> PELPEVETIRRTLLPLIVGKTIEDVRIFWPNIIRHPRDSEAFAARMIGQTVRGLERRGKFLKFLLDRDALISHLRMEGRYAVASALEPLEPHTHVVFCFTDGSELRYRDVRKFGTMHVYAKEEADRRPPLAELGPEPLSPAFSPAVLAERAVKTKRSVKALLLDCTVVAGFGNIYVDESLFRAGILPGRPAASLSSKEIERLHEEMVATIGEAVMKGQHHLYVYG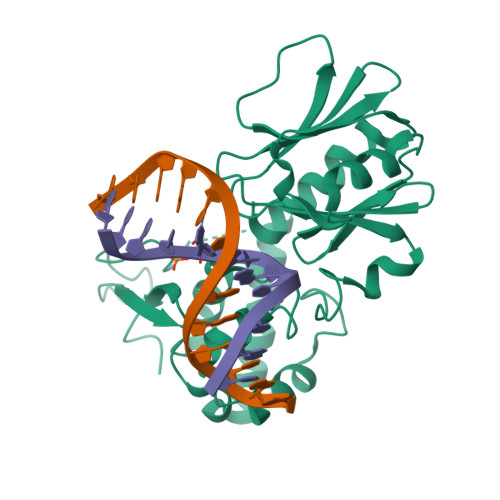RQGNPCKRCGTPIEKTVVAGRGTHYCPRCQR> DP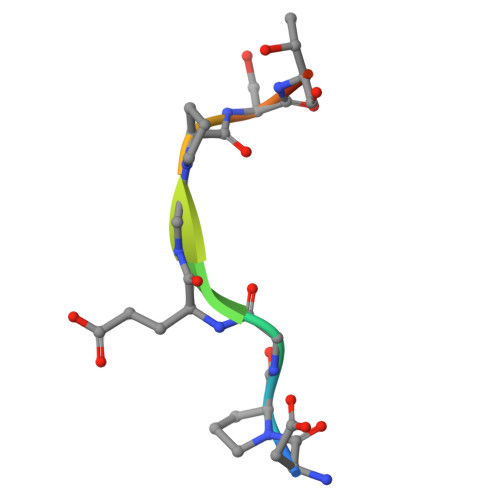GEGPSTGP> GGGAGUACGGUGAGGGUCGGGUCCAGUAGGUACGCCUACUGUUGAGUAGAGUG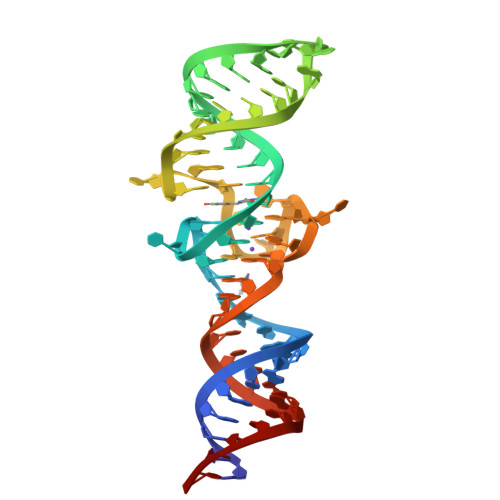UGGGCUCCGUACUCCC1-({(7M)-7-[1-(azetidin-3-yl)-6-chloro-1,2,3,4-tetrahydroquinolin-8-yl]thieno[3,2-b]pyridin-2-yl}methyl)pyrrolidine-2,5-dione | C24 H23 Cl N4 O2 S 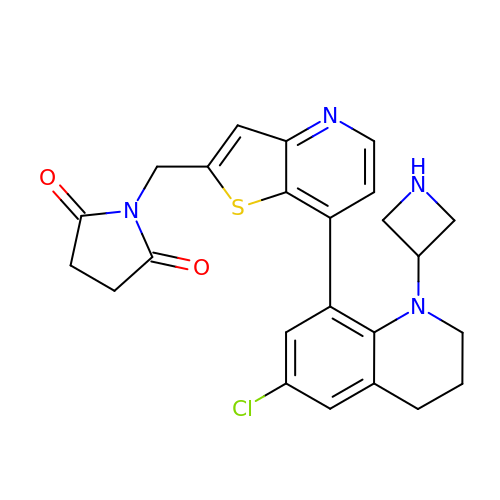| JLINGJINOLLCFE-UHFFFAOYSA-N>VNPCCYYPCQHQGICVRFGLDRYQCDCTRTGYSGPNCTIPEIWTWLRTTLRPSPSFIHFLLTHGRWLWDFVNATFIRDTLMRLVLTVRSNLIPSPPTYNIAHDYISWESFSNVSYYTRILPSVPRDCPTPMGTKGKKQLPDAEFLSRRFLLRRKFIPDPQGTNLMFAFFAQHFTHQFFKTSGKMGPGFTKALGHGVDLGHIYGDNLERQYQLRLFKDGKLKYQMLNGEVYPPSVEEAPVLMHYPRGIPPQSQMAVGQEVFGLLPGLMLYATIWLREHNRVCDLLKAEHPTWGDEQLFQTARLILIGETIKIVIEEYVQQLSGYFLQLKFDPELLFGAQFQYRNRIAMEFNQLYHWHPLMPDSFRVGPQDYSYEQFLFNTSMLVDYGVEALVDAFSRQPAGRIGGGRNIDHHILHVAVDVIKESRVLRLQPFNEYRKRFGMKPYTSFQELTGEKEMAAELEELYGDIDAL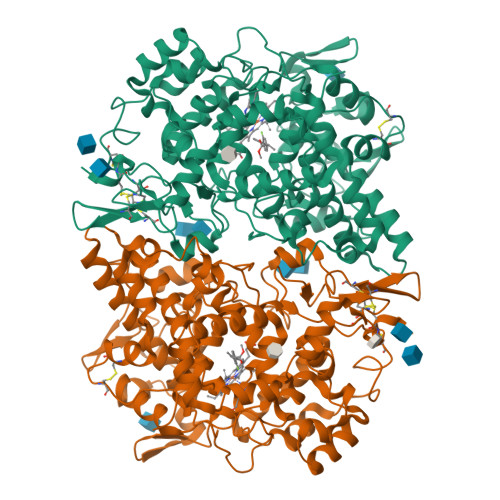EFYPGLLLEKCHPNSIFGESMIEMGAPFSLKGLLGNPICSPEYWKASTFGGEVGFNLVKTATLKKLVCLNTKTCPYVSFHVP[2x]>GPGMAVKHLIVLKFKDEITEAQKEEFIKTYVNLVNIIPAMKDVYWGKDVTQKNKEEGYTHIVEVTFESVETIQD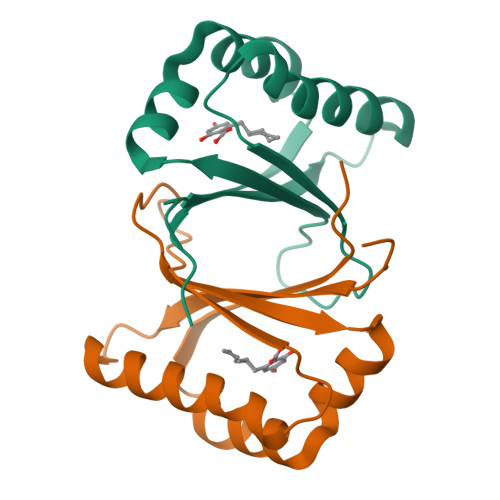YIIHPAHVGFGDVYRSFWEKLLIFDYTPRK[2x]> GAEGHIAHYDLNKLHSTSEAAVNKEHILILTPMQTFHQQYWDNLLQLNYPRELIELGFITPRTATGDLALKKLENAIKKVQTDKKTQRFSKITILRQNSQSFDKLMEKERHALDVQKERRAAMALARNELLFSTIGPHTSWVLWLNADIIETPPSLIQDMTKHNKAILAANIYQRFYDEEKKQPSIRPYDFNNWQESDTGLEIASQMGDDEIIVEGYAEIATYRPLMAHFYDANGVPGEEMALDGVGGGCTLVKAEVHRDGAMFPNFPFYHLIETEGFAKMAKRLNYDVFGLPNYLVYHIEEENH

The ScMnn9 glycosyltransferase is essential for the formation of mannosylated proteins that form mannan in the yeast cell wall. The synthesis of mannoproteins starts by the extension of the α-1,6-linked mannose to form a backbone of at least 10 α-1,6-linked mannose residues. This reaction is carried out by the M-Pol I heterodimeric complex, composed of the mannosyltransferases ScMnn9p and ScVan1p. ScMnn9p and ScVan1p belong to the CAZy glycosyltransferase family GT-62. This family contains metal-dependent, retaining mannosyltransferases that are predicted to possess the GT-A fold and use GDP-Man as their donor substrate.

The ScMnn9 structure was solved by a 2.2 Å single-wavelength anomalous dispersion (SAD) phasing experiment with a mercury derivative and refined against 2.0 Å synchrotron diffraction data of a mutant (D236N) in the presumed GT-A DxD catalytic motif, in complex with GDP and Mn2+, yielding a final R/Rfree of 0.19/0.24. The structure reveals that ScMnn9, and by extension the entire GT-62 glycosyltransferase family, adopts the GT-A fold as previously proposed by sequence analysis. Seven β-strands form a sheet that is covered on both sides by α-helices. However, ScMnn9 has a unique hairpin loop formed by two additional β-strands (I262-N283). The loop could potentially act as a molecular ruler for the formation of a mannose backbone of defined length or act as a guide to recognize and correctly position protein N-linked glycans for mannosyl transfer. The metal is coordinated by a histidine side chain, a carboxylate and the pyrophosphate moiety of GDP. The carboxylate metal ligand is part of the canonical GT-A fold DxD motif. Both the α- and β-phosphates of the GDP interact with the metal, similar to the RmMGS enzyme. Despite the fact that ScMnn9-D236N was soaked or co-crystallized with GDP-Man, electron density for mannose was not observed. ScMnn9 D236 is the first aspartic acid in the canonical GT-A DxD catalytic motif, and mutation to the isosteric asparagine results in the loss of activity, similar to the previously reported less conservative D236A mutation.> MLNFIPKRCPSVSLLFGKRPVQRIEVGQARHQLEIPVETIEKIYE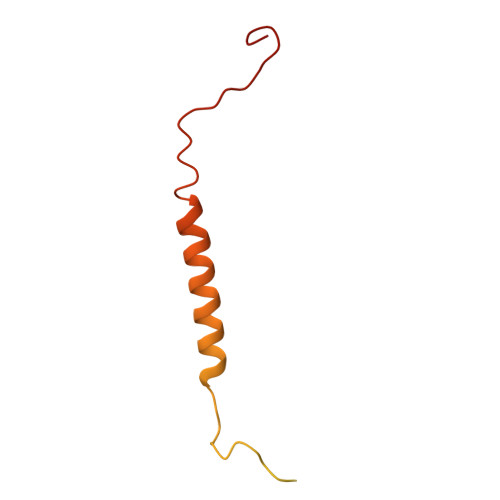GVDSRLEYHNKDYNAMKWKDFMKLKLDAYHLLEASQSETAAKSALSDLNWFSDLADIYSGQQTMAEMDVALKAQGEQKLSYPIQGKNIK>SNAMSENKMKALPFLSMSNLNLHNKRVMIREDLNVPMKNGKITNDERIVRALPTIQKAIEQKARVMILSHLGRPEEGKFEKEFSLAPVARLLSKKLNQKVPLINDWLKGVAVEPGQAILCENVRFNKGENENNTELAKRMAELCDIFVMDAFATAHRAQASTAGVAAYAKLACAGPLLISEVEALSRALENPQKPLVAVVGGSKVSTKIHLLENLLDKVDQLIVGGGIANTFLKAQGYSIGKSLCENEWLDAAQQFWEKAAEKNVSLPLPVDVIVADELSEDAKATVKNIDAVTSNESIFDVGPNTSATYAKLMAQAGTIVWNGPIGVFEIEAFSQGTRALAQAVAKSTAYSIVGGGDTLAALDKFNLTDQM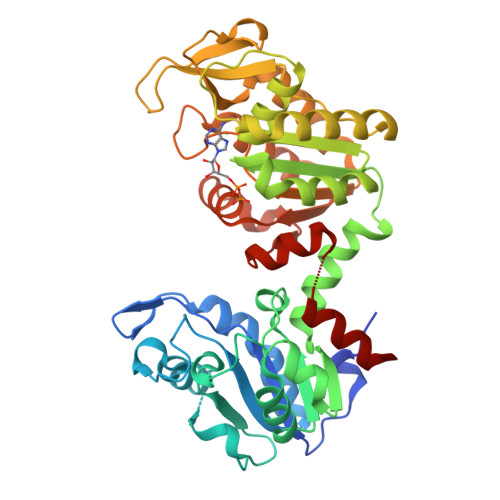SYVSTAGGAFLEFLEGKILPAIKILTQRAKEY[3x]> SLDIQSLDIQCEELSDARWAELLPLLQQCQVVRLDDCGLTEARCKDISSALRVNPALAELNLRSNELGDVGVHCVLQGLQTPSCKIQKLSLQNCCLTGAGCGVLSSTLRTLPTLQELHLSDNLLGDAGLQLLCEGLLDPQCRLEKLQLEYCSLSAASCEPLASVLRAKPDFKELTVSNNDINEAGVRVLCQGLKDSPCQLEALKLESCGVTSDNCRDLCGIVASKASLRELALGSNKLGDVGMAELCPGLLHPSSRLRTLWIWECGITAKGCGDLCRVLRAKESLKELSLAGNELGDEGARLLCETLLEPGCQLESLWVKSCSFTAACCSHFSSVLAQNRFLLELQISNNRLEDAGVRELCQGLGQPGSVLRVLWLADCDVSDSSCSSLAATLLANHSLRELDLSNNCLGDAGILQLVESVRQPGC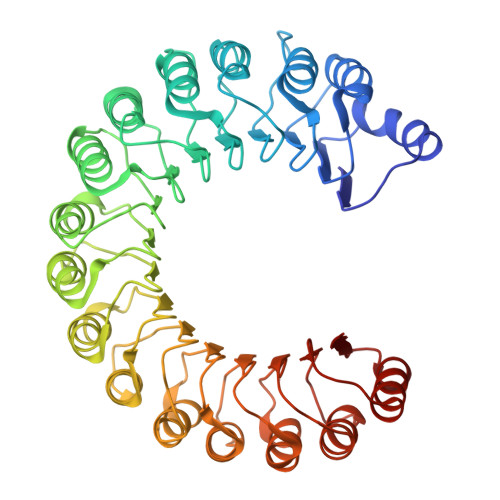LLEQLVLYDIYWSEEMEDRLQALEKDKPSLRVIS2-methylpropyl 2-acetamido-2,4-dideoxy-alpha-L-threo-hex-4-enopyranosiduronic acid | C12 H19 N O6 | 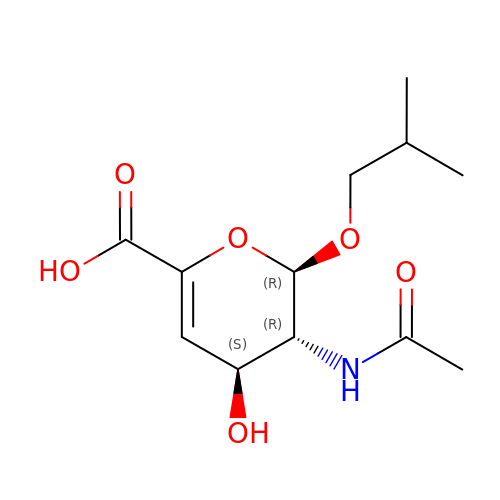QDVFOADQCFRSSP-MKPLZMMCSA-N> YAADWDGVPVPANPGSGKTWELHPLSDDFNYEAPAAGKSTRFYERWKEGFINPWTGPGLTEWHPHYSYVSGGKLAITSGRKPGTNQVYLGSITSKAPLTYPVYMEARAKLSNMVLASDFWFLSADSTEEIDVIEAYGSDRPGQEWYAERLHLSHHVFIRDPFQDYQPTDA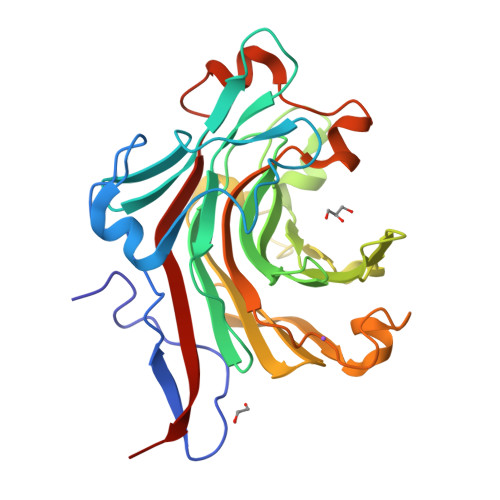GSWYADGKGTKWRDAFHRVGVYWRDPWHLEYYVDGKLVRTVSGQDIIDPNGFTGGTGLSKPMYAIINMEDQNWRSDNGITPTDAELADPNRNTYYVDWVRFYKPVPINGNAT4-[(3S)-1-AZABICYCLO[2.2.2]OCT-3-YLAMINO]-3-(1H-BENZIMIDAZOL-2-YL)-6-CHLOROQUINOLIN-2(1H)-ONE 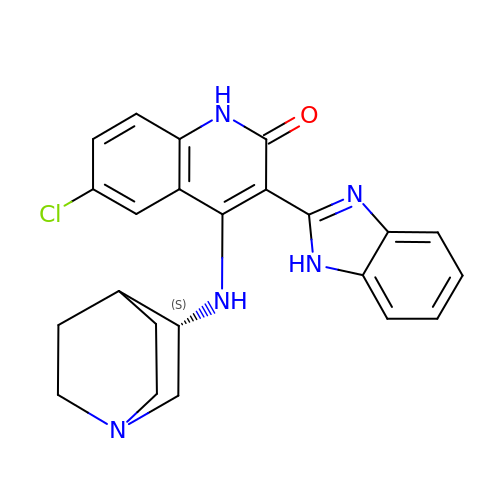| C23 H22 Cl N5 O | MOVBBVMDHIRCTG-LJQANCHMSA-N> MVDMAVTPVALLEASHLHYHVQQQALINDVSLHIASGEMVAIIGPNGAGKSTLLRLLTGYLSPSHGECHLLGQNLNSWQPKALARTRAVMRQYSELAFPFSVSEVIQMGRAPYGGSQDRQALQQVMAQTDCLALAQRDYRVLSGGEQQRVQLARVLAQLWQPQPTPRWLFLDEPTSA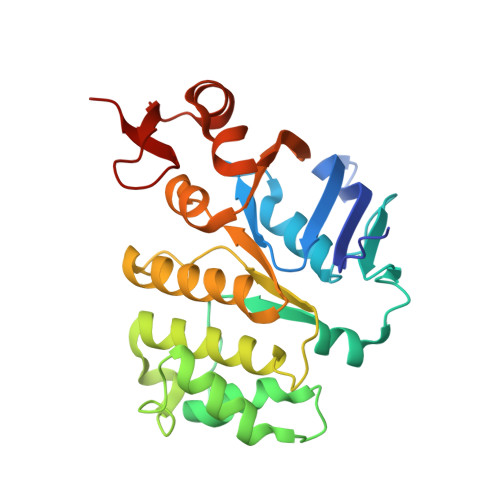LDLYHQQHTLRLLRQLTRQEPLAVCCVLHDLNLAALYADRIMLLAQGKLVACGTPEEVLNAETLTQWYQADLGVSRHPESALPQIYLRQ>[3x]MNHLPVVGEDYVEIPDGRPFAPLAGKIEVVEIFGYTCPHCAHFDSKLQAWGARQAKDVRFTLVPAVFGGVWDPFARAYLAADVLGVAKRSHTAM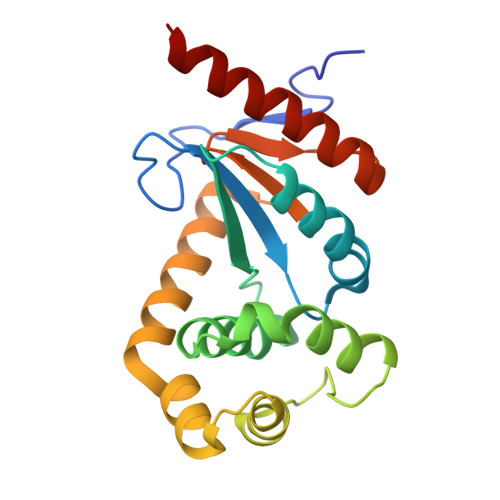FEAIHEKGSVPIQNVGPDELAVFYAGYGVQPDRFVATFNGPEVEKRFQAARAYALKVRPVGTPTIVVNGRYMVTGHDFEDTLRITDYLVSRERAASHGR(2Z,4Z)-2-imino-6-oxohex-4-enoic acid | C6 H7 N O3 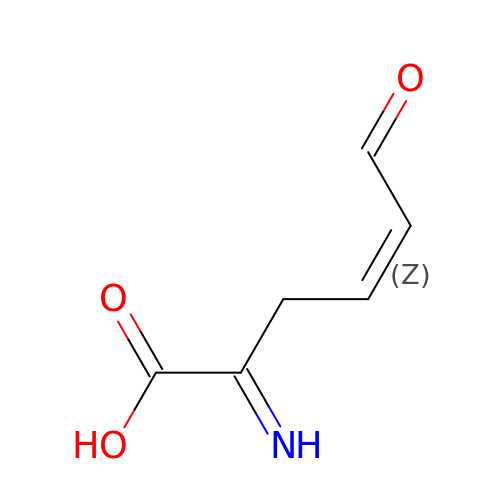| IZBQCPKKCVTOTK-PQZOIKATSA-N As a sirtuin (SIR2) family protein, defense-associated sirtuin2 (DSR2) has been demonstrated to participate in bacterial anti-phage resistance via depleting nicotinamide adenine dinucleotide (NAD+) of infected cells, which can be activated by tail tube protein (TTP) and inhibited by DSR anti-defense 1 (DSAD1) of diverse phages. To defend phage invasion, Bacillus subtilis utilizes DSR2 proteins to sense and recognize phage SPR tail tube protein (TTP), then unleashes NADase activity of its SIR2 domain to deplete the cell of NAD+ and abort phage propagation during infection. Each DSR2 protomer contains three domains, an N-terminal SIR2 domain (SIR2, residues 1 to 297), a middle connector domain (MID, residues 297 to 627), and a C-terminal sensor domain (CTD, residues 627 to 1005). Structural analyses and biochemical studies reveal that DSR2 forms a tetramer with a SIR2 central core and two distinct conformations.

To elucidate underlying mechanisms, the cryo-EM structure of the DSR2-DSAD1 complex has been determined at 2.98 Å, with DSAD1 bound to DSR2A in the open state. In the structure, DSAD1 consists of strands β1 to β5 and one α helix between β4 and β5. Extensive interactions between DSAD1 and DSR2open consist of residues S18, I53, C57, D58, F59, E76, F79, and F81 of DSAD1 and residues K960, R802, W919, K965, N963, N863, S909, and S908 of DSR2open. In addition, the binding of DSAD1 introduces new contact with DSR2closed by DSAD1 residues K6, Y16, and S18 forming hydrogen bonds with DSR2closed residues S637 and I631 of CTD and residues G572 and Y574 of the MID. Compared to TTP binding of DSR2, the DSAD1 binding induces much slighter conformational change with an RMSD of 1.138 Å between the overall structures of the DSR2-DSAD1 complex and apo DSR2. Although the SIR2 domains within the DSR2-DSAD1 complex exhibit conformational twisting to a certain extent, the magnitude of twist is much smaller compared to the changes induced by TTP binding. This conformational change on the SIR2 domain tetramer is not harsh enough to hurt proper tetramerization conformation critical for its NADase activity. When superimposing TTP and DSAD1 simultaneously in one protomer, DSAD1 binds to DSR2open with the lifting α42 generating a wider binding pocket; the falling of α42 in the closed state clearly blocks the entry of DSAD1 like a door bolt. With the direct steric hindrance in the binding site occupied by DSAD1, it is impossible for TTP to bind to the same DSR2 protomer. The binding of DSAD1 locks DSR2open in the resting state, by not only competitively occupying the binding pocket but also stabilizing the MID of the adjacent protomer to stop the transduction of TTP-induced conformational changes in DSR2closed, allosterically inhibiting the activation on DSR2 NADase activity triggered by TTP binding.

>MVKVDLESKRYGEKLKEVFLMLDNNVVECIKEITESSRNGKLVFFVGAGVSTLSDYPQWWRLVDKYHEELYGSPKKGNYSSDEYLRIPQIFYNVKGEMAFDGILKDFFQVDKPTNPIHDKILAMNPAHVITTNYDNLIDTACWKRGKYFSVISAEEDVANATSSRYLLKVAGDFRKGFKGENVVLKEDDYLNYDQNYPLISNLMKTIIATHTIVFIGYGLGDYNINMLLNWVRKLQKDSFHKPFFIRTDPSPIENETLIYYENKGLRIIDAASLIDSNEYDYLERYSAVMDLLIESQENKFITKDDEVIDYIYGKISPLFALQYIRKIDLKHVFEYDYHFEVNGTVVRHKNKGFGYMERFFELKESCDERSKLSKKQYERFNALFNFFEKNGVICMAKDAGTLNTSIEINSLAYHGKYDVMKKFIEEQSVSIEDDYKKAFFLACLGRWEESYDLYSNIILNSIDESNGCVYYLSQINRYRIYQSITQAVTQFNGLGLLTFGRHYKPFTDEFLARIEREMTNFNIDDLFNGMPFEFQKKYKILEFLSDNQFLYDDTVKLFELTNKVRSEMSEGSYSFGMSSDIVVLLRLYDNLRFLYENCLWSVSFHEFHQYIRNSMSLLIEKAEYERTRDIDELGFSFFGKKSGFFMEYYDFVNISRHFKIDDIKNLERSCSIDKIRFGEQEKIEEYLVGIAEEITKQFSANGMNVVFYTQFISEAKAALYFAKYVKLSEEGLGKIVKALLFYFPERDLDIGKRYVWLERLTKCNELPKSIISIIDDFLVLQAEKHIDQNYSEVSSNGLYSRDYGALIKHFEKNFISKRLSEITLCLTQDKQKQIDFLFKLLPLLSTNAKSHLLSFKSVENINDLMNGIRIGLIDEFTPEHEELIIEYLETRKVNYIVEKEKGIQTFSSNDYMSTFGIWYFLEEINNSKMEEFIGMDDQYDFFVDPENFDYKKFIPSWLKNYNDKLLGKIAGNKHMKHHVIEVLKERVKNSNDKRYLEILMNYFI[4x];> KDTGATHDLVYHSKINTFVWDVEFDIVLSDSKELNKCYFVKCFNPYRINGKCDFAVSSIDIFSEGKRLLIENEFNFKITKAVHVATSKDVTEIVLHLSERISSPFPIVKEVVYLD YerA from Bacillus subtilis is considered a novel class of enzymes that are capable of catalyzing the deamination of 6mA to produce hypoxanthine. YerA is the first identified binuclear metal-dependent enzyme that specifically catalyzes the hydrolytic deamination of 6mA, representing a novel class of deaminases. Additionally, YerA has been shown to possess conserved key amino acid residues that form a binuclear metal center. Our deamination assays showed that N6-methyladenosine (N6-mAdo) served as a more favorable substrate than its base derivative 6mA.

Here, we report the high-resolution structure of the C-terminal region of YerA, which exhibited a compact architecture composed of two antiparallel β-sheets with no obvious close structural homologs in Protein Data Bank. Despite extensive trials, only two constructs pET-28a(+)/YerAAla15-Arg580 and pET-28a(+)/YerAGly380-Arg580 successfully produced crystals, after removing the N-terminal 6 × His affinity tag. While the former construct produced poor-diffracting crystals, pET-28a/YerAGly380-Arg580 readily crystallized with a cubic morphology in ammonium sulfate or potassium phosphate as the precipitants. The cubic crystals belonged to a tetragonal system, with the space group P41212, and each asymmetric unit contains one molecule with an estimated solvent content of 51%. Continuous and well-defined electron density was observed for the entire polypeptide chain, except for the first two residues introduced by cloning. The refined model comprised 201 amino acids and 101 water molecules, with refinement statistics summarized in Table 1. The YerAGly380-Arg580 structure adopts an α+β fold with a globular shape, divisible into two domains: an N-terminal β-sheet of eight antiparallel strands flanked by helices (Gly380-Leu550) and a C-terminal β-sheet featuring three antiparallel strands (Gln551-Arg580). These domains are spatially close, forming a compact structure devoid of central cavities or concave surfaces. Analysis by the PISA server indicated that YerAGly380-Arg580 does not form an oligomeric structure within the crystal lattice. A DALI search for YerAGly380-Arg580 homologs retrieved only remotely related structures with RMSD scores generally ranging from ~5 Å or above, with 70–90 aligned Cαs, indicating that the domain’s structure is unique. Attempts to express various YerA constructs without this domain invariably rendered the remaining enzyme insoluble, suggesting a structural role. During the structural comparison of YerA’s Gly380-Arg580 domain with MAPDA, we found that this domain may function as a lid covering YerA’s active site, presumably playing an equivalent role to MAPDA’s α4-helix.

> GGLVPLELSYDMTMDDLQFSMPMGVKMRNAVIMEPYMIEIDNSMEQLSFDHDESYLTMLDRHGKWRVNTMIKGFASSVQGFVSSFTTTGDIVAIGKNKADMLLAFARMKEIGGGIVLAENGNILHEIPLALCGCASSEAYEDVLEKEQKLRDLLTERGYEFCDPIYTLLFLQSTHLPYIRITPRGIFDVMKKTVLFPSIMR>[2x]HGYVSAYENGVAEGRATLCRVP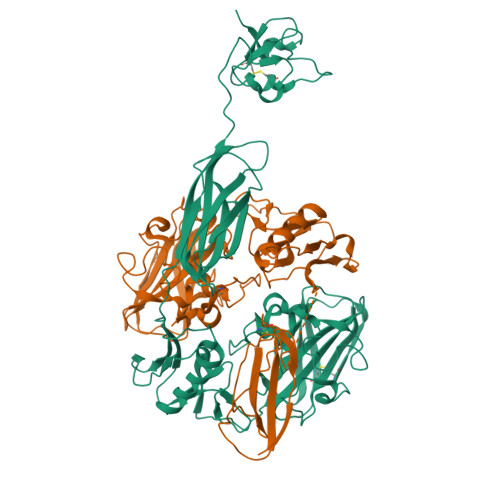ANDTNEKNTNCGGIEYEPQSVEGPDGFPETGPRDGKIASAENSLAAALDEQTADRWVKRPIQSGNQHFEWNFTANHITKDWKYYITKADWNPNQPLARDSFDLNPFCVVDGGMVKPPMRVSHLCNVPEREGYQVILAVWDVGDTAASFYNVIDVKFDGDSPVLPDWNQGGQIYPSQDLNVGDSVYTRVFGQNGENVSYSTELVIDSEELGAANNWSHALATKINQEQTMLQAGQLNAEGVISPIYGTNPIYLKQGSGLKNVEIDYKINSTAPEYDLEVYGLESEYIIGDSATQLDLTLEATGDIKTEMTVYNHHHESLSSHSAELSDGQVEAATMTLSKSEPGHHMLVVVVKDQQGKVIEQNTLDFHLIEEQTPPPSGEYDFVFPEGLNTYTAGTKVLASDGAVYQCKEFPFSGYCTQWSPSATQFEPGKGSHWSEAWNKVN> AVQGTSQFTCFYNSRAQISCVWSQDGALQDTSCQVHA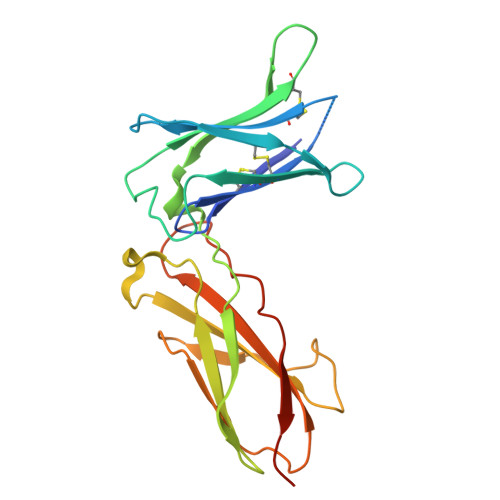WPDRRRWQQTCELLPVSQASWACNLILGAPDSQKLTTVDIVTLRVLCREGVRWRVMAIQDFKPFENLRLMAPISLQVVHVETHRCNISWEISQASHYFERHLEFEARTLSPGHTWEEAPLLTLKQKQEWICLETLTPDTQYEFQVRVKPLQGEFTTWSPWSQPLAFRTKPAALGKDT We used de novo protein design to generate very closely related proteins that adopt two very different states—a short state and a long state, like a viral fusion protein—and then created a single molecule that can be found in both forms. Inspired by class I viral fusion proteins, such as influenza hemagglutinin, we chose homotrimeric helical bundles as the fundamental architecture. We decided on a design scheme with two divergent conformations containing a constant six-helix bundle “base” and a variable portion with three inner helices and three “flipping” helices. In the compact “short” state (∼66 Å height), the flipping helices fold back to interact with the inner helices; in the extended “long” state (∼100 Å height), they extend to form interactions with each other.

The interaction energy between the flipping helix and the inner helices in the short state was tuned by combining hydrogen bond layers (“A”) or hydrophobic layers (“X”) in different orders in each of three possible positions. Designs were given three-letter names corresponding to the layers in order, starting at the hinge proximal position. Structure prediction calculations (Rosetta symmetric fold-and-dock) suggested that some layer combinations (such as XAX) would be more favorable for the short state than others (such as AAA) and that the short and long backbones states would be among the lowest-energy states of these systems. SEC-MALS measurements indicated that, in solution, XAX, XAA, and AAA were trimeric as expected; CD wavelength and temperature measurements for XAX, XAA, and AAA showed that the designs were helical and highly temperature stable. The number and position of the hydrogen bond networks appears to determine the state which is populated—designs with one network folding into the short state, with two networks, into a more dynamic short state, and with three networks, into the long state.

>[3x]GSHMGTEDLKYSLERLREILERLEENPSEKQIVEAIRAIVENNAQIVEAIRAIVENNAQIVENNRAIIENNEAIGGGTKQLEEMKKQLKDLKRSLERG>MNAEDVKGFFASRESLDMEQYLVLDYYLESVGDIETALAHFCSEQSTAQWKRVGVDEDFRLVHAAKVIDYEVIEELEQLSYPVKHSETGKIHACRVT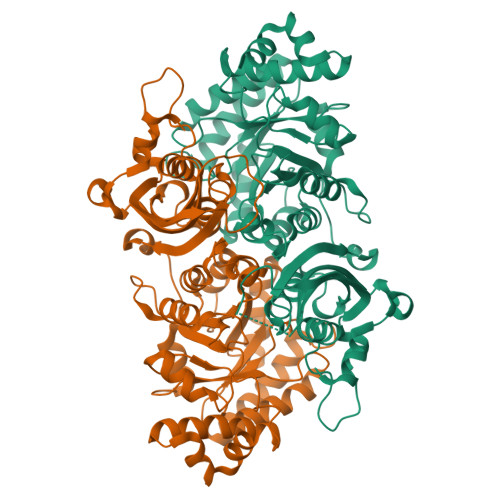IAHPHCNFGPKIPNLLTAVCGEGTYFTPGVPVVKLMDIHFPDTYLADFEGPKFGIEGLRDILNAHGRPIFFGVVKPNIGLSPGEFAEIAYQSWLGGLDIAKDDEMLADVTWSSIEERAAHLGKARRKAEAETGEPKIYLANITDEVDSLMEKHDVAVRNGANALLINALPVGLSAVRMLSNYTQVPLIGHFPFIASFSRMEKYGIHSKVMTKLQRLAGLDAVIMPGFGDRMMTPEEEVLENVIECTKPMGRIKPCLPVPGGSDSALTLQTVYEKVGNVDFGFVPGRGVFGHPMGPKAGAKSIRQAWEAIEQGISIETWAETHPELQAMVDQSLLKKQD[2x]> MAGIAMKLATDREAAEGLGSHERAIKYLNQDYETLRNECLEAGALFQDPSFPALPSSLGFKELGPYSSKTRGIEWKRPTEICADPQFIIGGATRTDICQGALGDSWLLAAIASLTLNEEILARVVPLDQSFQENYAGIFHFQFWQYGEWVEVVVDDRLPTKDGELLFVHSAEGSEFWSALLEKAYAKINGCYEALSGGATTEGFEDFTGGIAEWYELRKPPPNLFKIIQKALEKGSLLGCSIDITSAADSEAVTYQKLVKGHAYSVTGAEEVESSGSLQKLIRIRNPWGQVEWTGKWNDNCPSWNTVDPEVRANLTERQEDGEFWMSFSDFLRHYSRLEICNLTPDTLTCDSYKKWKLTKMDGNWRRGSTAGGCRNYPNTFWMNPQYLIKLEEEDEDDEDGERGCTFLVGLIQKHRRRQRKMGEDMHTIGFGIYEVPEELTGQTNIHLSKNFFLTTRARERSDTFINLREVLNRFKLPPGEYVLVPSTFEPHKNGDFCIRVFSEKKADYQTVDDEIEANIEE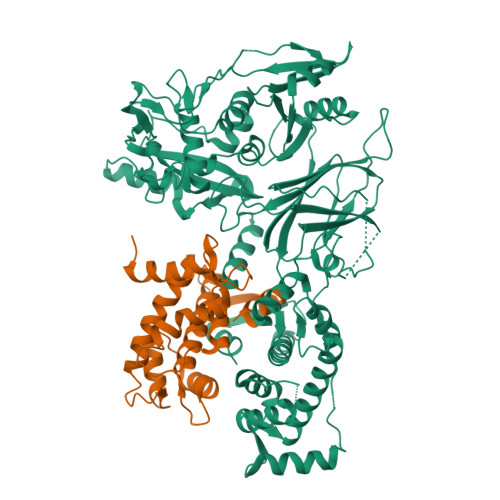IEANEEDIGDGFRRLFAQLAGEDAEISAFELQTILRRVLAKREDIKSDGFSIETCKIMVDMLDEDGSGKLGLKEFYILWTKIQKYQKIYREIDVDRSGTMNSYEMRKALEEAGFKLPCQLHQVIVARFADDELIIDFDNFVRCLVRLEILFKIFKQLDPENTGTIQLDLISWLSFSVL;> MHYSNIEANESEEERQFRKLFVQLAGDDMEVSATELMNILNKVVTRHPDLKTDGFGIDTCRSMVAVMDSDTTGKLGFEEFKYLWNNIKKWQGIYKRFDTDRSGTIGSNELPGAFEAAGFHLNQHIYSMIIRRYSDETGNMDFDNFISCLVRLDAMFRAFRSLDKNGTGQIQVNIQEWLQLTMYS> MQFLNMFFFDIYPYIAGAVFLIGSWLRYDYGQYTWRAASSQMLDRKGMNLASNLFHIGILGIFVGYFFGMLTPHWMYEAWLPIEVKQKMAMFAGGASGVLCLIGGVLLLKRRLFSPRVRATTTGADILILSLLVIQCALGLLTIPFSAQHMDGSEMMKLVGWAQSVVTFHGGASQHLDGVAFIFRLHLVLGMTLFLLFPF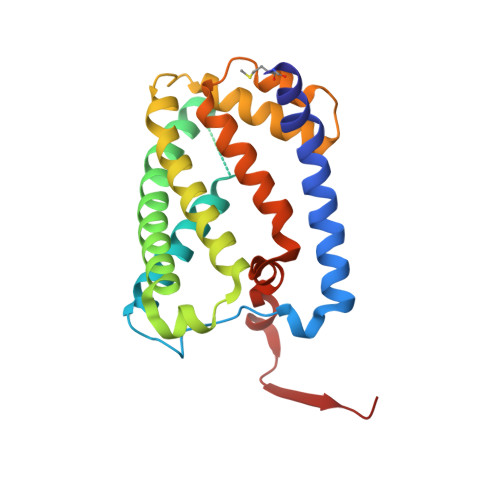SRLIHIWSVPVEYLTRKYQLVRARH> MRLLYLHADRFEYKTVKPALKNPPDPPGEASFGEALVVF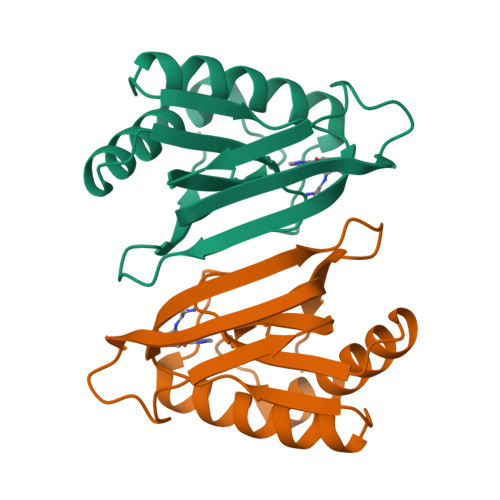TTVEDGDGPQTVMYAASDIASHSSRLKVTTVILYPYAHLSSRLAKPMAAHKRLIELEGALRTKFPGHVHRAPFGWYKSFSIACKGHPLAELSRSFTE> GSHMTYRDAATALEHLATYAEKDGLSVEQLMDSKTRGGLTYNDFLVLPGKIDFPSSEVVLSSRLTKKITLNAPFVSSPMDTVTEADMAIHMALLGGIGIIHHNCT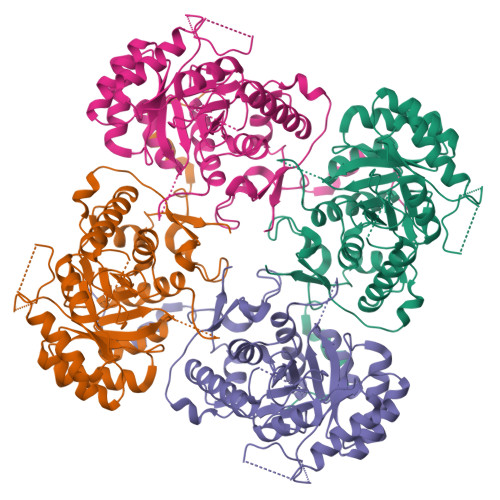AEEQAEMVRRVKKYENGSQDGPLASKSADTKQLLCGAAIGTIDADRQRLAMLVEAGLDVVVLDSSQGNSVFQINMIKWIKETFPDLQVIAGNVVTREQAASLIHAGADGLRIGMGSGSICITQEVMACGRPQGTAVYNVTQFANQFGVPCIADGGVQNIGHITKAIALGASTVMMGGMLAGTTESPGEYFFRDGKRLKTYRGMGSIDAMQKTDVKGNAATSRYFSESDKVLVAQGVTGSVIDKGSIKKYIPYLYNGLQHSCQDIGVRSLVEFREKVDSGSVRFEFRTPSAQLEGGVHNLHSYEKRLFD>VFHKIRNEDLIFNESLGQGTFTKIFKGVRREVGDYGQLH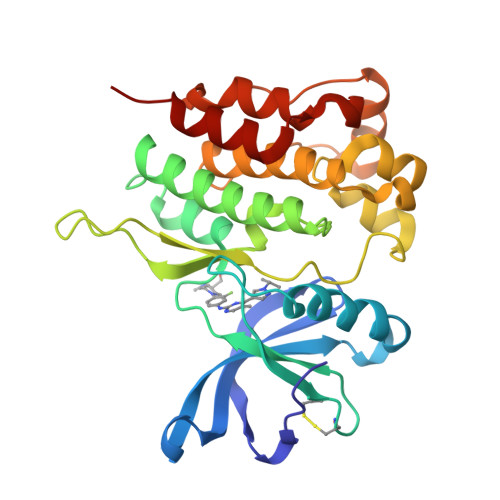ETEVLLKVLDKAHRNYSESFFEAASMMSKLSHKHLVLNYGVCFCGDENILVQEFVKFGSLDTYLKKNKNCINILWKLEVAKQLAWAMHFLEENTLIHGNVCAKNILLIREEDRKTGNPPFIKLSDPGISITVLPKDILQERIPWVPPECIENPKNLNLATDKWSFGTTLWEICSGGDKPLSALDSQRKLQFYEDRHQLPAPKAAELANLINNCMDYEPDHRPSFRAIIRDLNSLFT[2x]> GKAVIAIHGGAGAISRAQMSLQQELRYIEALSAIVETGQKMLEA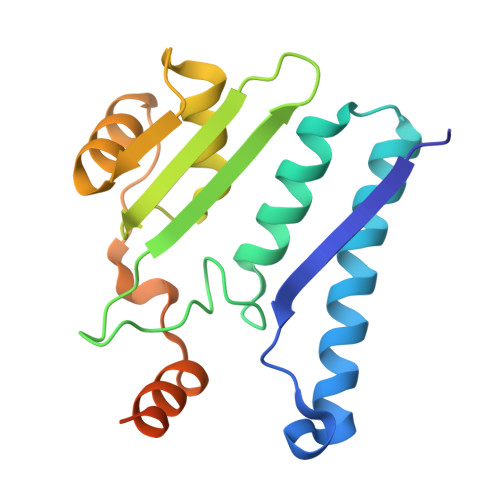GESALDVVTEAVRLLEECPLFNAGIGAVFTRDETHELDACVMDGNTLKAGAVAGVSHLRNPVLAARLVMEQSPHVMMIGEGAENFAFARGMERVSPEIFSTSLRYEQLLAARKEGATVLDHSGAPLDEKQKMG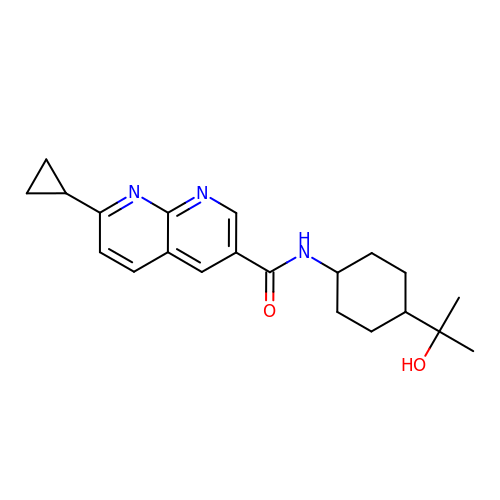7-cyclopropyl-N-[trans-4-(2-hydroxypropan-2-yl)cyclohexyl]-1,8-naphthyridine-3-carboxamide | C21 H27 N3 O2 | VEKOTFOGNGVLSE-QAQDUYKDSA-N> GSPGIRMSLKSDEVFAKIAKRLESIDPANRQVEHVYKFRITQGGKVVKNWVMDLKNVKLVESDDAAEATLTMEDDIMFAIGTGALPAKEAMAQDKMEVDGQVELIFLLEPF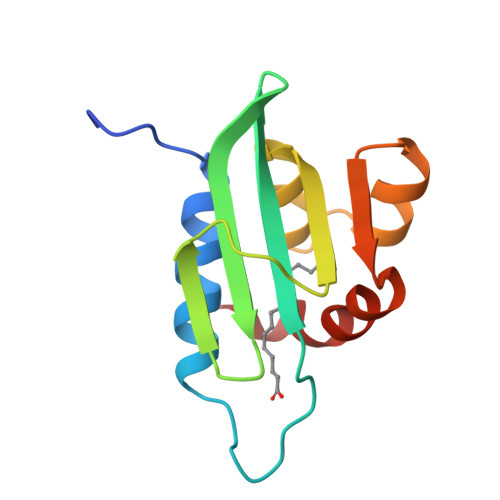IASLK>MGHHHHHHHHHHHHSSGHIDDDDKHMLEMIQSHPLLAAPLAVGDTIGFFSSSAPATVTAKNRFFRGVEFLQRKGFKLVSGKLTGKTDFYRSGTIKERAQEFNELVYNPDITCIMSTIGGDNSNSLLPFLDYDAIIANPKIIIGYSDTTALLAGIYAKTGLITFYGPALIPSFGEHPPLVDITYESFIKILTRK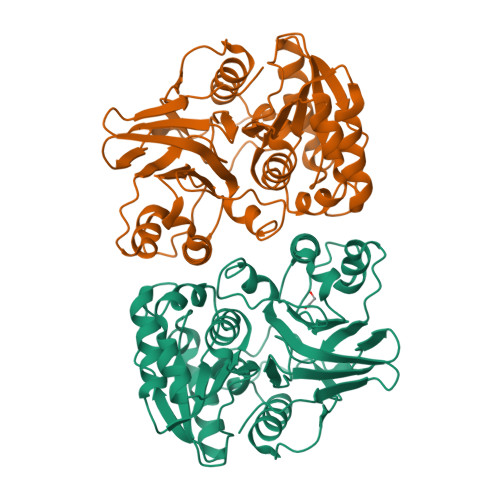QSGIYTYTLPEKWSDESINWNENKILRPKKLYKNNCAFYGSGKVEGRVIGGNLNTLTGIWGSEWMPEIRNGDILFIEDSRKSIATVERLFSMLKLNRVFDKVSAIILGKHELFDCAGSKRRPYEVLTEVLDGKQIPVLDGFDCSHTHPMLTLPLGVKLAIDFDNKNISITEQYLSTEK[2x]>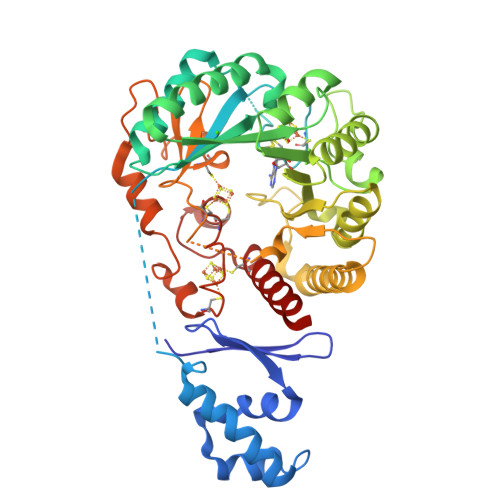SNAMAMIHKFSMMGTNIVVDVNSGAVHVVDDISFDILDYYKNFTAGEIKNKLAHKYNADEIDEALREIESLEAEGLLFSEDPYKEYVSSMDRKSVVKALCLHISHDCNLRCKYCFASTGNFGGQRNMMSLEVGKKAIDFLISESGNRKNLEIDFFGGEPMMNFDVVKGIIEYARQKEKEHNKNFRFTLTTNGLLLNDENIKYINENMQNIVLSIDGRKEVNDRMRIRIDGSGCYDDILPKFKYVAESRNQDNYYVRGTFTRENMDFSNDVLHLADEGFRQISVEPVVAAKDSGYDLREEDLPRLFEEYEKLAYEYVKRRKEGNWFNFFHFMIDLTQGPCIVKRLTGCGSGHEYLAVTPEGDIYPCHQFVGNEKFKMGNVKEGVLNRDIQNYFKNSNVYTKKECDSCWAKFYCSGGCAANSYNFHKDINTVYKVGCELEKKRVECALWIKAQEM[2x]Here, we report an arthropod-conserved insect chitinase belonging to group III from the pest Ostrinia furnacalis (OfChtIII), which contains two GH18 domains that act without synergism according to enzymatic assays and structural investigations. OfChtIII contains 987 amino-acid residues and is composed of four domains: a predicted TM domain (residues 7–29), two catalytic domains, GH18A (residues 94–461) and GH18B (residues 530–889), and a CBM14 domain (residues 922–976). The two GH18 domains of OfChtIII possess similar structures and substrate specificities, which differentiate them from the chitinolytic chitinase OfChtI-CAD. The degradation activity of GH18A and GH18B (or GH18B-CBM14) in combination towards EGC was equal to the activity calculated from the sum of the individual activities, suggesting that there was no synergistic effect between them.

GH18B crystallized in space group P41212 and its structure was determined by molecular replacement using the structure of human AMCase as a template. To study the substrate-binding mode, the structures of two complexes of GH18B were crystallized and obtained: that of wild-type GH18B complexed with (GlcNAc)3 and that of the GH18B-E647L mutant with a bound (GlcNAc)5. These structures were resolved to resolutions of between 2.2 and 2.8 Å, and all data-collection and structure-refinement statistics are summarized in Table 3. Secondly, the structures of GH18A and GH18B are very similar, with an r.m.s.d. of 0.88 Å for 344 Cα atoms. Although the overall structures of GH18A and GH18B are similar to that of OfChtI-CAD, with r.m.s.d.s of 1.3 Å (for 367 Cα atoms) and 1.5 Å (for 360 Cα atoms), respectively, there are obvious differences between the two enzymes. Firstly, GH18A and GH18B from OfChtIII do not have the same surface hydrophobic planes as found in the GH18 domain of OfChtI (characterized by Phe159, Phe194, Trp241 and Tyr290). Secondly, both GH18 domains have shorter and shallower substrate-binding clefts than OfChtI-CAD. As calculated by the CASTp software with default parameters, the volumes of the substrate-binding clefts of OfChtI-CAD, GH18A and GH18B were estimated to be 1628, 1399 and 1100 Å3, respectively.

> EPQVLCYLTSWSSKRPSAGRFMPENVDPTLCTHVIYAFATLKDHKLTEADEKDADMYDKVVALREKNPNLKILLAIGGWAFGSTPFKELTSNVFRMNQFVYEAIEFLRDYQFNGLDVDWEYPRGADDRAAFVSLLKELRLAFEGEAKTSGQPRLLLTAAVPASFEAIAAGYDVPEISKYLDFINVMTYDFHGQWERQVGHNSPLFPLESATSYQKKLTVDYSAREWVRQGAPKEKLMIGMPTYGRSFTLINDTQFDIGAPASGGGQAGRFTNEAGFMSYYEICEFLREDNTTLVWDNEQMVPFAYREDQWVGFDDERSLKTKMAWLKEEGFGGIMVWSVDMDDFRGSCGTGKYPLITAMKQELSGYKVKLEYDGPYESSSPTGQYTTKDPHEVTCEEEDGHISYHKDHADCTMYYMCEGERKHHMPCPSNLVFNPNENVCDWPENVEGCQQHTQAPAAKR> MSLSDLLYEIQDKVGLLTMNRISKHNAFDNQLLTEMRIRLDSAINDTNVRVIVLKANGKHFSAGADLTWMQSMANFTEEENLEDSLVLGNLMYSISQSPKPTIAMVQGAAFGGGAGLAAA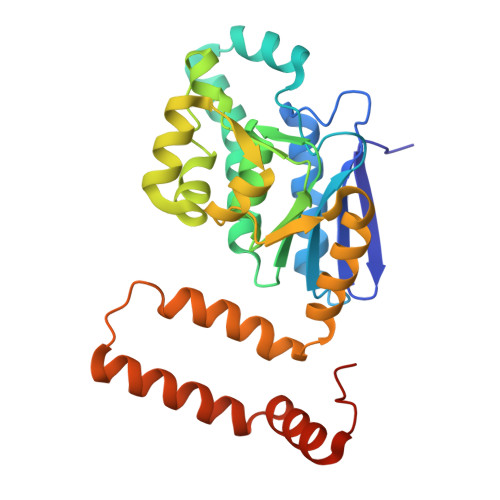CDIAIASTSARFCFSEVKLGLIPAVISPYVVRAIGERAAKMLFMSAEVFDATRAYSLNLVQHCVPDDTLLEFTLKYASQISNNAPEAVKNSKQLAQYVANKKIDEELVRYTASLIAHKRVSDEGQEGLKAFLNKEIPNWNEGHHHHHH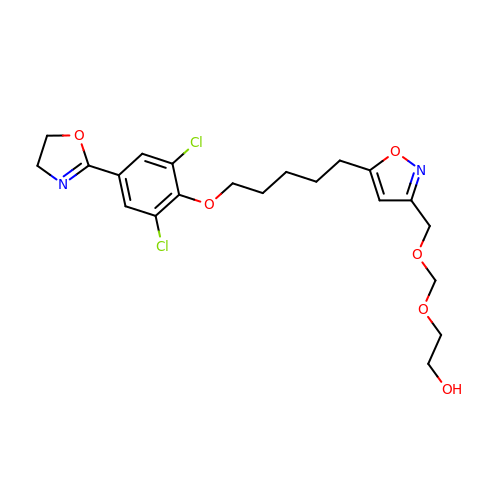5-(5-(2,6-DICHLORO-4-(4,5-DIHYDRO-2-OXAZOLYL)PHENOXY)PENTYL)-3-(HYDROXYETHYL OXYMETHYLENEOXYMETHYL) ISOXAZOLE | C21 H26 Cl2 N2 O6 | JLSNWEWWUSOSMP-UHFFFAOYSA-N> MGRKKIQIQRITDERNRQVTFTKRKFGLMKKAYELSVLCDCEIALIIFNHSNKLFQYASTDMDKVLLKYTEYNEPHESR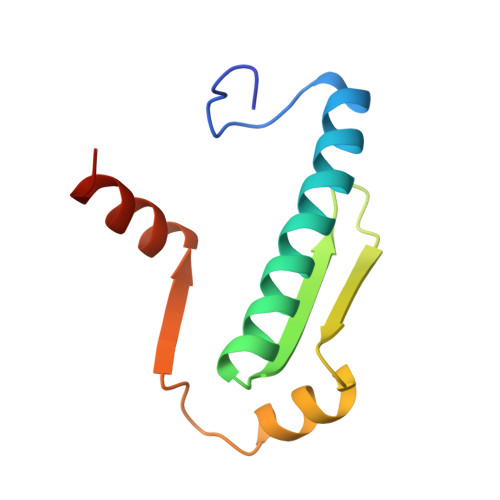TNADIIETLRKKGFNG> GSHMTPKDDEFYQQWQLKYPKLILREASSVSEELHKEVQEAFLTLHKHGCLFRDLVRIQGKDLLTPVSRILIGNPGCTYKYLNTRLFTVPWPVKGSNIKHTEAEIAAACETFLKLNDYLQIETIQALEELAAKEKANEDAVPLCMSADFPRVGMGSSYNGQDEVDIKSRAAYNVTLLNFMDPQKMPYLKEEPYFGMGKMAVSWHHDENLVDRSAVAVYSYSCEGPEEESEDDSHLEGRDPDIWHVGFKISWDIETPGLAIPLHQGDCYFMLDDLNATHQHCVLAGSQPRFSSTHRVAECSTGTLDYILQRCQLALQNVCDDVDNDDVSLKSFEPAVLKQGEEIHNEVEFEWLRQFWFQGNRYRKCTDWWCQ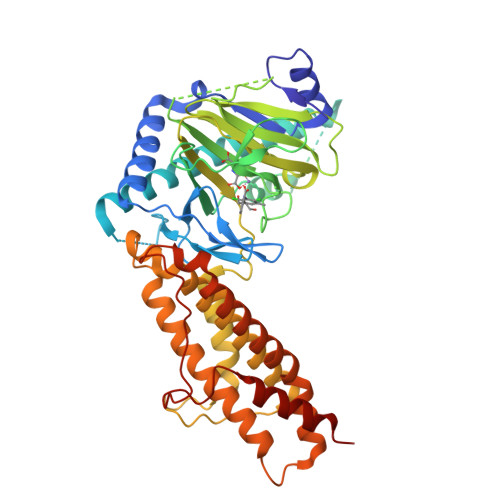PMAQLEALWKKMEGVTNAVLHEVKREGLPVEQRNEILTAILASLTARQNLRREWHARCQSRIARTLPADQKPECRPYWEKDDASMPLPFDLTDIVSELRGQLLEA> TTEQ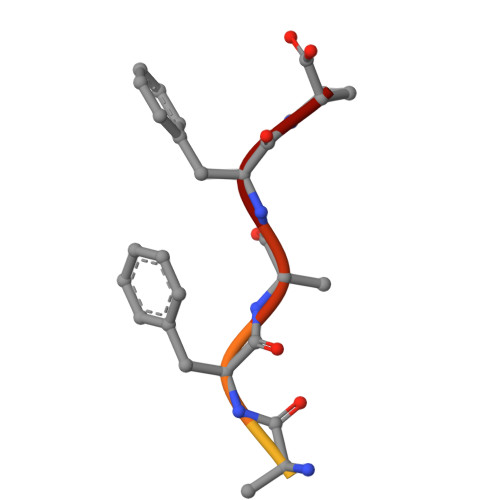SDFKFP>[2x]FEFPEELKTKLQEHINYFPKKRQAILLCLHEIQNYYGYIPPESLKPLADMLELPLNHVEGVVAFYDMFDREDKAKYRIRVCVSIVCHLMGTNKLLKALENILGIKPGEVTPDGKFKIVPVQCLGACSEAPVFMVNDDEYKFESEVQLNEILSRYT;>[2x]RSYPAIPRIYAETTLNMLLKRAKKPRVHSIDEYLKDGGYQALEKALNMSPEEIIDWVDKSTLRGRGGAGFPTGKKWKFAVQNPGPRYFICNADEMEPGTFKDRIIIERDPHLLIEGIIISSYAIGANEAYIYIRGEYPAGYYILRDAIEEAKKKGFLGKNILGSGFDLEIYVARGAGAYICGEETALIESLEGKRGHPRLKPPYPVQKGLWGKPTVVNNVETIANVPFIISMGWEEYRYIGPSDYAGPKLFPVSGKVKKPGVYELPMNTTLREVIFKYAGGTLGNKKVKAVFSGALDCFSSEELDIPMDYSPLGFGGTGTVIVLTEEDDIVEAALKIAEFYEHETCGQCTPCRVGCYEQANLLEKIYKGEATEQDWEGFDFVNRNIQPTSICGLGAVAGRLIRQTLEKFPEEWEKYRK

Complex I couples the transfer of two electrons from NADH to ubiquinone (Q) with the translocation of four protons across the membrane. The L-shaped complex is structured into a peripheral arm that protrudes into the aqueous milieu and catalyzes electron transfer with one FMN and 8–10 iron–sulfur ([Fe–S]) clusters, and a membrane arm embedded in the lipid bilayer that mediates proton translocation. We have determined structures of the electron-input module of complex I from the hyperthermophilic bacterium Aquifex aeolicus, encompassing subunits NuoE and NuoF that contain the FMN cofactor, the [4Fe–4S] cluster N3, and the [2Fe–2S] cluster N1a, respectively, both in the air-oxidized and dithionite-reduced states at resolutions up to 1.8 Å. Here, we show that the redox state of N1a regulates NADH oxidation in complex I by inducing a conformational change close to the NADH-binding site.

To ensure that the methionine residue at the homologous position in the E. coli complex does not change the local structure, we generated, purified, and crystallized the A. aeolicus S96MF variant. The mutation did not impose any substantial structural changes, although the hydroxyl group of the original S96 is no longer available for hydrogen bonding to the peptide carbonyl of D94. In addition, the larger side chain of the methionine residue displaces two water molecules, while another water molecule shows up in a different position. Still, the flip of the peptide bond upon reduction of the S96MF variant is clearly detectable. Accordingly, statements on the A. aeolicus enzyme can be extrapolated to the one from E. coli.>[4x]MHSLMKPTREPQINLFKKSNPYKAKVISNVLLTPETGTGKRPKKEGEALVHRIVLAIDHSAYPYVIGQSGGVIPPGEDPEKKAKGLADVGYTVRLYSIASPSYSFGMKEDNIEFIIKRDNIYDENGNIQFKGVC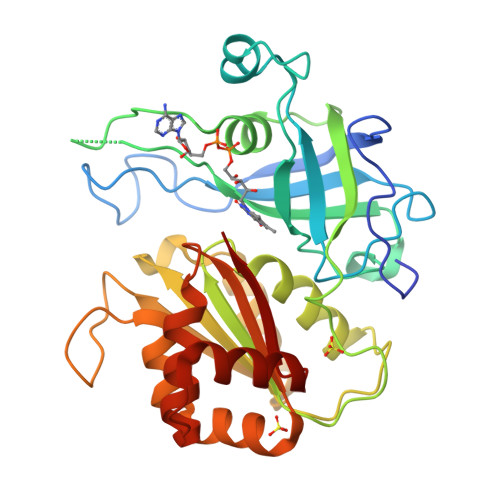SNYMCDLKPGDEVTMTGPSGKKFLLPNTDFSGDIMFLATGTGIAPFIGMSEELLEHKLIKFTGNITLVYGAPYSDELVMMDYLKGLESKHKNFKLITAISREEKNSFDGGRMYISHRVREQAEAVKKILNGGGRFYICGGPKGMEKGVIEEIQKISGNTGTYEEFKHHLEGAHQLFVETY> MQVNRLPFFTNHFFDTYLLISEDTPVGSSVTQLLARDMDNDPLVFGVPGEEASRFFAVEPDTGVVWLRQPLDRETKSEFTVEFSVSDHQGVITRKVNIQVGDVNDNAPTFHNQPYSVRIPENTPVGTPIFIVNATDPDLGAGGSVLYSFQPPSPFFAIDSARGIVTVIQELDYEVTQAYQLTVNATDQDKTR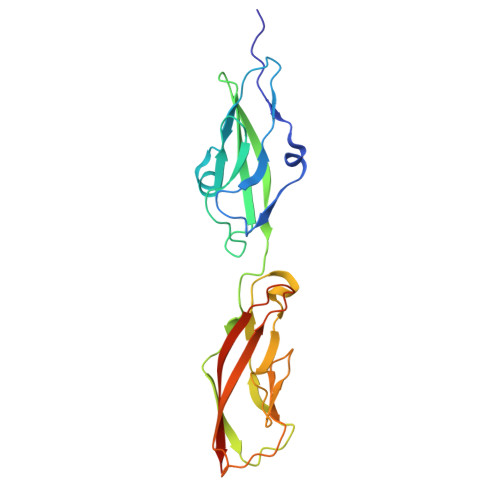PLSTLANLAIIITDLEHHHHHH benzyl-N-[(2S)-1-[[(3S)-7-amino-1-(benzylamino)-1,2-dioxoheptan-3-yl]amino]-5-(2-methyl-2-phenylhydrazinyl)-1,5-dioxopentan-2-yl]carbamate | C34 H42 N6 O6 | 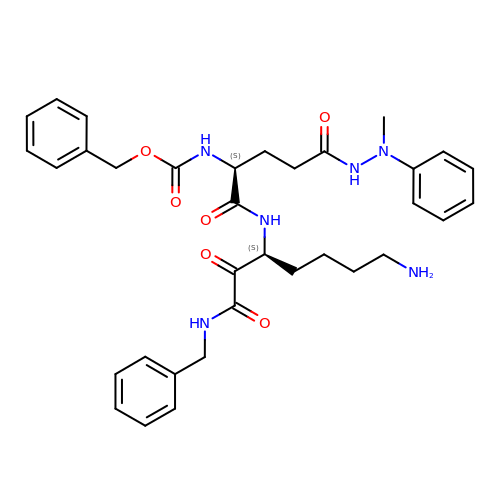XDVSKHGOOXWVDB-VMPREFPWSA-N> APDTSVSNKQNFSTDVIYQIFTDRFSDGNPANNPTGAAFDGT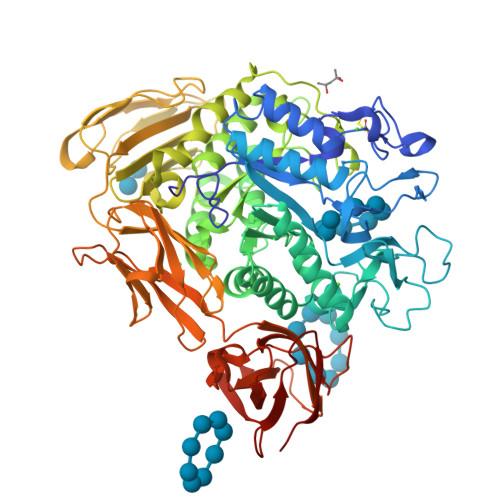CTNLRLYCGGDWQGIINKINDGYLTGMGVTAIWISQPVENIYSIINYSGVNNTAYHGYWARDFKKTNPAYGTIADFQNLIAAAHAKNIKVIIDFAPNHTSPASSDQPSFAENGRLYDNGTLLGGYTNDTQNLFHHNGGTDFSTTENGIYKNLYDLADLNHNNSTVDVYLKDAIKMWLDLGIDGIRMNAVKHMPFGWQKSFMAAVNNYKPVFTFGQWFLGVNEVSPENHKFANESGMSLLDFRFAQKVRQVFRDNTDNMYGLKAMLEGSAADYAQVDDQVTFIDNHDMERFHASNANRRKLEQALAFTLTSRGVPAIYYGTEQYMSGGTDPDNRARIPSFSTSTTAYQVIQKLAPLRKCNPAIAYGSTQERWINNDVLIYERKFGSNVAVVAVNRNLNAPASISGLVTSLPQGSYNDVLGGLLNGNTLSVGSGGAASNFTLAAGGTAVWQYTAATATPTIGHVGPMMAKPGVTITIDGRGFGSSKGTVYFGTTAVSGADITSWEDTQIKVKIPAVAGGNYNIKVANAAGTASNVYDNFEVLSGDQVSVRFVVNNATTALGQNVYLTGSVSELGNWDPAKAIGPMYNQVVYQYPNWYYDVSVPAGKTIEFKFLKKQGSTVTWEGGSNHTFTAPSSGTATINVNWQP> MDKCKKVYENYPVSKCQLANQCNYDCKLK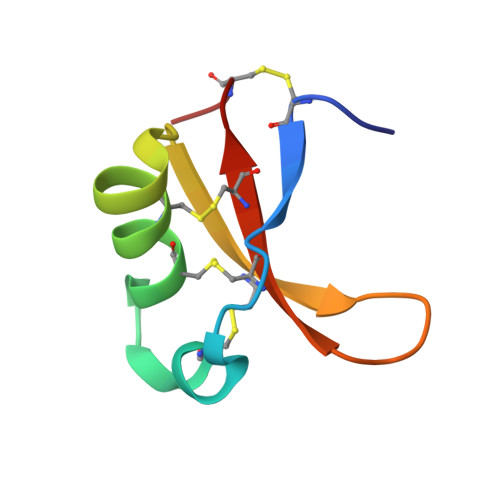KHARSGECFYDEKRNLQCICDYCEY>MHHHHHHENLYFQGHMKKWGDMFTWGVSTSSYQIEGAANQGGRGPSIWDTFSKIPGAVANGDNGDVACDHYHRYNEDLDLMKWLGVGAYHFSIAWPRVIPSGYGALNKEGMDFYDRLIDGALERGITPWPTLYHWDLPQSLQDKGGWNNRDCAYWFAEYSQKMAEAFSDRLKNWITINEPFCSAWLGHLYGVMAPGIKDLKTGINASHHLLLGHGLATKAIREVSSELKVGITLNFTPAITLGESSEDKLAVELADGFDNRWFGDPVFKAKYPEDIVKAFGKEVPIHPGDMEIISTPLDYLGLNYYFRQTVEYDATAKPLPYKQVTAPNVERTGMGWEVHAQSFTELLERVSKEYKPKEIFITENGSAWDDEVVDGKVDDPNRVSYLERHLDAMFAAKNKGVPISGYFAWSLIDNFEWAYGYAKRFGIIYVDYQTQKRIPKSSAYYYQKRIKESG[3x]

Here we report, in contrast, on a naturally occurring mutation of an otherwise invariant residue in the β-glucosidase BglM-G1 that balances a trade-off between structural stability and enzyme activity. β-glucosidases are enzymes hydrolyzing β-glycosidic bonds in substrates ranging from glycosides, to glucosylated flavonoids, glucosylceramides, and oligosaccharides, releasing nonreducing terminal glucosyl residues (see Ketudat et al. for a comprehensive review). They are also one of the key enzymes in the bioconversion of cellulosic material. The otherwise invariant arginine at position 75 changed to a histidine in this protein, while the other 36 amino acids deemed necessary for the function and structural integrity of members of this protein family remained unchanged. Our data indicate that the natural mutation to histidine at position 75 leads to the loss of an extensive electrostatic network, including a salt bridge in the active site region and implies that evolution of BglM-G1 traded a decrease in thermal stability for improved catalytic efficiency.

The fact that BglM-G1 evolved to be a fully active β-glucosidase with a naturally occurring substitution of the otherwise invariant arginine at position 75 provided us with the unique opportunity to study the structural implications of this amino acid in β-glucosidases. Based on size-exclusion chromatography, which showed that both proteins exist in a monomeric form in solution, we assume that the trimeric assembly in the crystal is packing-generated. Comparison of the structures of BglM-G1 and TmGH1 monomers revealed a root mean square deviation (RMSD) value of 0.53 Å over 313 Cα atoms and the conformation of the active site glutamates were highly similar. Upon solving the structure, we observed both in wild type and H75R an unresolved electron density within the active site tunnel. This density does not seem to originate from a peptide chain and we were not able to fit an atomic structure to it. There was, however, a major difference in electrostatic interactions between the mutation site and the active site nucleophile. The naturally occurring histidine at position 75 in BglM-G1 formed only a single hydrogen bond with the backbone oxygen of threonine 116, while arginine at position 75 formed, in addition to hydrogen bond interactions with residues Gln163 and Thr116, a salt bridge with the catalytic nucleophile glutamate at position 349 Fig. 2 CD spectroscopic analysis and X-ray crystal structure of BglM-G1 and its H75R variant. We then determined the melting temperature of both proteins by monitoring changes in ellipticity at 222 nm, while continuously increasing the temperature from 10 to 80 °C. For BglM-G1 the mid-point of transition was at 51.4 °C (324.6 K with a 95% confidence interval between 324.4 and 324.8 K), while the melting temperature of H75R was at 54.9 °C (328.1 K with a 95% confidence interval between 328.9 and 329.2 K).THIENO[2,3-B]PYRIDINE-2-CARBOXAMIDINE 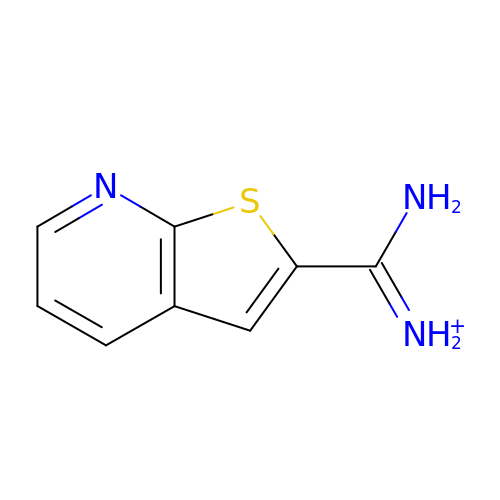| C8 H8 N3 S | GZEJMYFXZMUAEC-UHFFFAOYSA-O>[2x]MTIKLIVGLANPGAEYAATRHNAGAWYVDLLADRHRAPL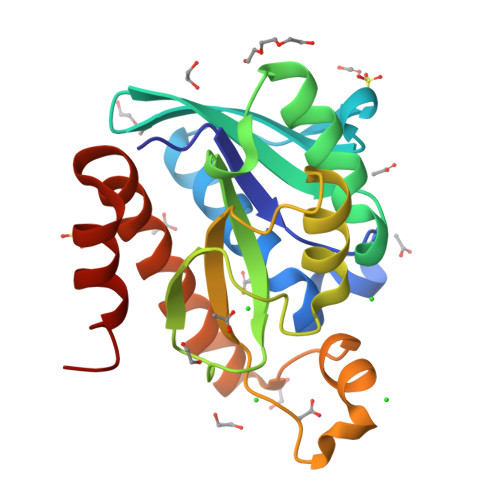REESKFFGYTSRINLAGEDVRLLVPTTFMNLSGKAVAAMATFYRINPDEILVAHDELDLPPGVAKFKLGGGHGGHNGLKDIISKLGNNPNFHRLRVGIGHPGDKNKVVGFVLGKPPASEQKLIDDAVDEAARCTEILLKDGLTKATNRLHAFKAQ> DEEFPEQKAGEVINQPMMMAARQLHDEARKWSSKGNDIIAAAKRMALLMAEMSRLVRGGSGTKRALIQCAKDIAKASDEVTRLAKEVAKQCTDKRIRTNLLQVCERIPTISTQLKILSTVKATM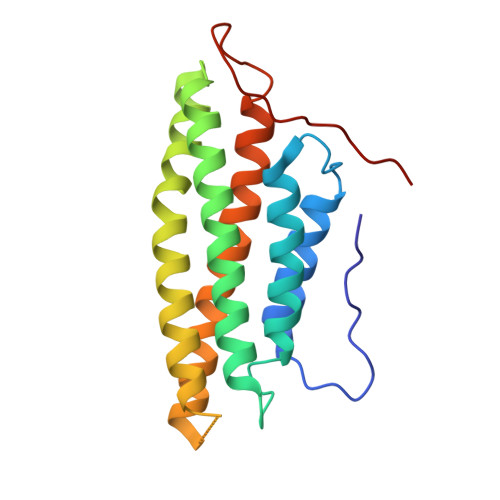LGRTNISDEESEQATEMLVHNAQNLMQSVKETVREAEAASIKIRTDAGFTLRWVRKTPWYQ> LYF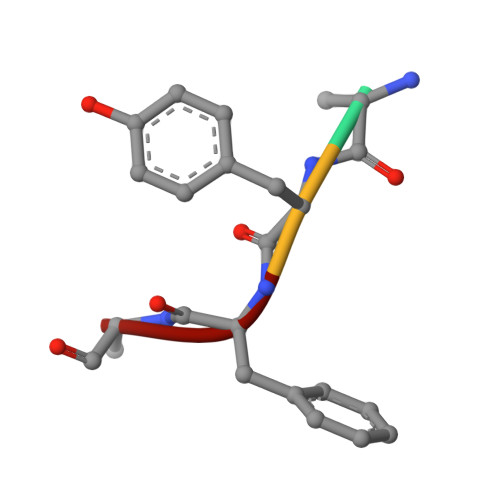A>MNLIPTVIETTNRGERAYDIYSRLLKDRIIMLGSQIDDNVANSIVSQLLFLQAQDSEKDIYLYINSPGGSVTAGFAIYDTIQHIKPDVQTICIGMAASMGSFLLAAGAKGKRFALPNAEVMIHQPLGGAQGQATEIEIAANHILKTREKLNRILSE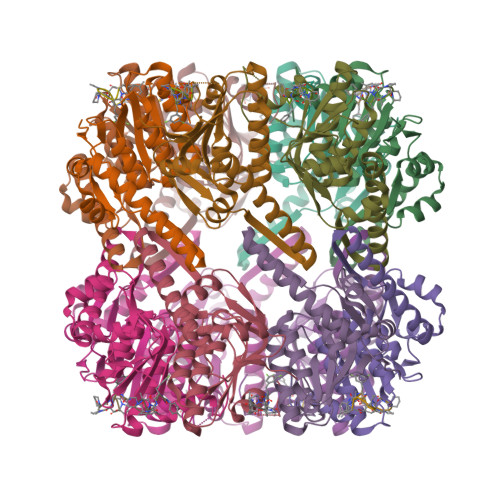RTGQSIEKIQKDTDRDNFLTAEEAKEYGLIDEVMVPETKLEHHHHHH[14x]>GGEVPIGDPKELNGMEIAAVYLQPIEMEPRGIDLAASLADIHLEADIHALKNNPNGFPEGFWMPYLTIAYELKNTDTGAIKRGTLMPMVADDGPHYGANIAMEKDKKGGFGVGNYELTFYISNPEKQGFGRHVDE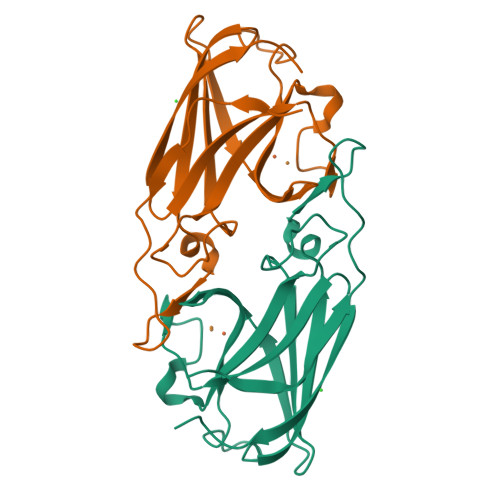ETGVGKWFEPFKVDYKFKYTGTPK[2x]>[2x]MSPLRKTVPEFLAHLKSLPISKIASNDVLTICVGNESADMDSIASAITYSYCQYIYNEGTYSEEKKKGSFIVPIIDIPREDLSLRRDVMYVLEKLKIKEEELFFIEDLKSLKQNVSQGTELNSYLVDNNDTPKNLKNYIDNVVGIIDHHFDLQKHLDAEPRIVKVSGSCSSLVFNYWYEKLQGDREVVMNIA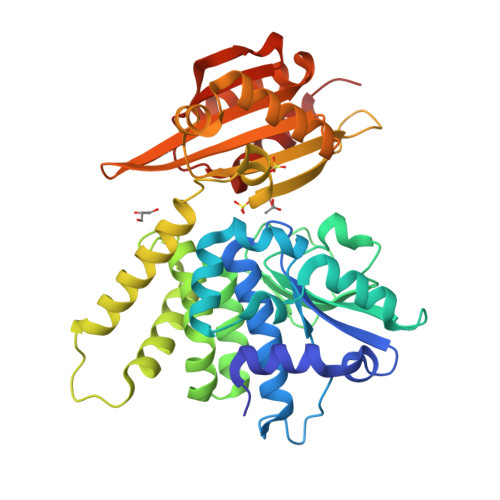PLLMGAILIDTSNMRRKVEESDKLAIERCQAVLSGAVNEVSAQGLEDSSEFYKEIKSRKNDIKGFSVSDILKKDYKQFNFQGKGHKGLEIGLSSIVKRMSWLFNEHGGEADFVNQCRRFQAERGLDVLVLLTSWRKAGDSHRELVILGDSNVVRELIERVSDKLQLQLFGGNLDGGVAMFKQLNVEATRKQVVPYLEEAYSNLEE> GKKAWCWASYLEEEKAVAVPAKLFKEHQSFPYNKNGFKVGMKLEGVDPEHQSVYCVLTVAEVCGYRIKLHFDGYSDCYDFWVNADALDIHPVGWCEKTGHKLHPPKGYKEEEFNWQTYLKTCKAQAAPKSLFENQNITVIPSGFRVGMKLEAVDKKN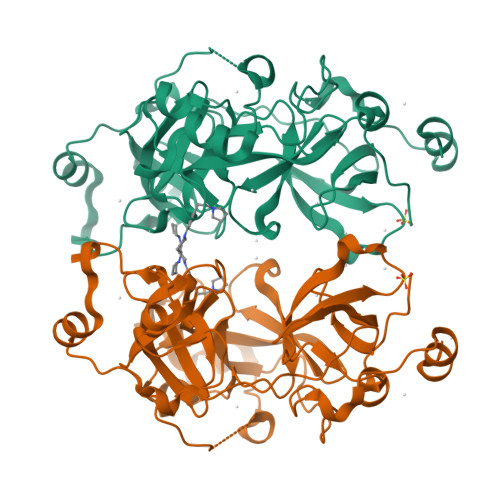PSFICVATVTDMVDNRFLVHFDNWDESYDYWCEASSPHIHPVGWCKEHRRTLITPPGYPNVKHFSWDKYLEETNSLPAPARAFKVKPPHGFQKKMKLEVVDKRNPMFIRVATVADTDDHRVKVHFDGWNNCYDYWIDADSPDIHPVGWCSKTGHPLQPPL>NATEIRASVGKMIDGIGRFYIQMCTELKLSDYEGRLIQNSLTIERMVLSAFDERRNKYLEEHPSAGKDPKKTGGPIYRRVDGKWRRELILYDKEEIRRIWRQANNGDDATAGLTHMMIWHSNLNDATYQRTRALVRTGMDPRMCSLMQGSTLPRRSGAAGAAVKGVGTMVMELIRMIKRGINDRNFWRGENGRRTRIAYERMCNILKGKFQTAAQRTMVDQVRESRNPGNAEFEDLIFLARSALILRGSVAHKSCLPACVYGSAVASGYDFEREGYSLVGIDPFRL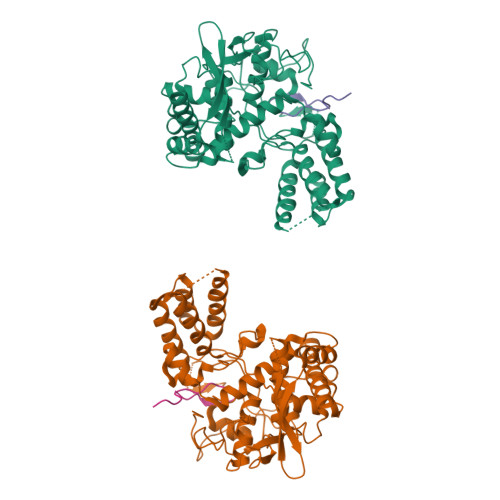LQNSQVYSLIRPNENPAHKSQLVWMACHSAAFEDLRVSSFIRGTKVVPRGKLSTRGVQIASNENMETMESSTLELRSRYWAIRTRSGGNTNQQRASSGQISIQPTFSVQRNLPFDRPTIMAAFTGNTEGRTSDMRTEIIRLMESARPEDVSFQGRGVFELSDEKATSPIVPSFDMSNEGSYFF[2x];>SSGQISIQPTFSVQRNLPF[2x]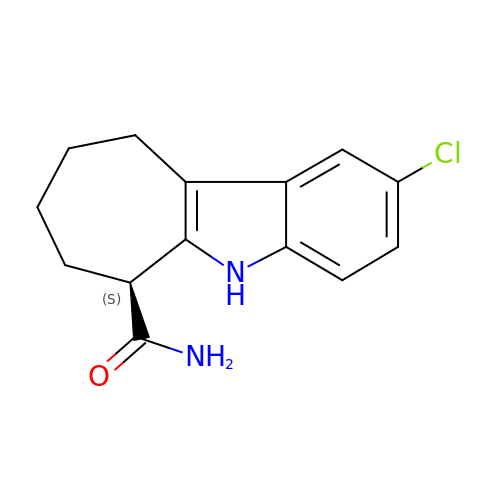(6S)-2-chloro-5,6,7,8,9,10-hexahydrocyclohepta[b]indole-6-carboxamide | C14 H15 Cl N2 O | ABIVOOWWGYJNLV-JTQLQIEISA-N>GSMAQNAEKDTLIVASKVKAYIKSKGFMTSGDAVDGLNEKLYALIDDALK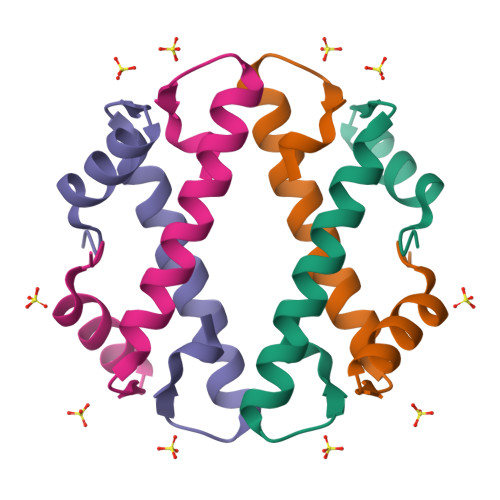RTESNKRTTVRPTDF[2x]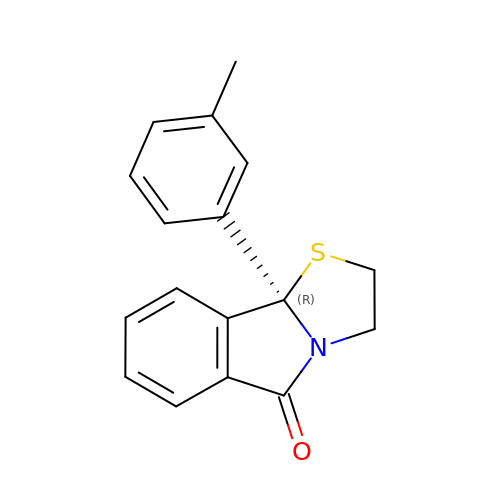(R)-(+)9B-(3-METHYL)PHENYL-2,3-DIHYDROTHIAZOLO[2,3-A]ISOINDOL-5(9BH)-ONE | C17 H15 N O S | FQVDJZWFSZSGGA-QGZVFWFLSA-N> MGETKKMICLVDGEHYFPVVKDSIEILDDLEHIDVVAVVFIGGTEKLQIEDPKEYSEKLGKPVFFGPDPKKIPYDVIKKCVKKYNADIVMDLSDEPVVDYTKRFRIASIVLKEGAVYQGADFKFEPLTEYDVLEKPSIKIIGTGKRIGKTAVSAYAARVIHKHKYNPCVVAMGRGGPREPEIVEGNKIEITAEYLLEQADKGVHAASDHWEDALMSRILTVGCRRCGGGMLGDTFITNVKRGAEIANKLDSDFVIMEGSGAAIPPVKTNRQIVTVGANQPMININNFFGPFRIGLADLVIITMCEEPMATTEKIKKVEKFIKEINPSANVIPTVFRPKPVGNVEGKKVLFATTAPKVVVGKLVNYLESKYGCDVVGVTPHLSNRPLLRRDLKKYINKADLMLTELKAAAVDVATRVAIEAGLDVVYCDNIPVVIDESYGNIDDAIIEVVEMAIDDFKNNR

The enzyme cyclic di-phosphoglycerate synthetase that is involved in the production of the osmolyte cyclic 2,3-diphosphoglycerate has been studied both biochemically and structurally. The reaction involves the transfer of the γ-phosphate group from ATP to the substrate 2,3 -diphosphoglycerate and the subsequent SN2 attack to form a phosphoanhydride. The unique structure of cDPGS is made up of an N-terminal domain which is crucial for the stabilization of the active dimeric structure and the ligand interactions, and a C-terminal domain that contains a P-loop kinase fold as part of its structure. Since the cDPGS reaction is exergonic at cellular concentrations, cDPG accumulation is favored thermodynamically until this reaction reaches equilibrium. cDPG appears to play a role in the thermoprotection of proteins, and increased thermostability has been demonstrated for several model enzymes in its presence.

The cDPGS crystallized readily in many screening conditions and the structure of the apo-cDPGS was solved by the single wavelength anomalous dispersion (SAD) method using data collected from a selenomethionine protein crystal. The space group was determined to be I222 with a single protomer of cDPGS in the asymmetric unit. The structure was refined to 1.7 Å resolution and was found to contain the entire polypeptide chain. This has been refined to R and Rfree values of 17.7 and 21.3%, respectively. The structure of cDPGS can be split into two domains. The smaller N-terminal domain contains a six-stranded β-sheet of mixed type with direction + + + + + − and connectivity -1x,-1x,3x,1x,1 flanked by 4 α-helices (α1–α4). The β-sheets of the two N-terminal domains in the cDPGS dimer form a large intersubunit 12 strand β-sheet on the molecular dyad. The larger C-terminal domain (residues 136–460) contains a twelve-stranded β-sheet (β7 – β18) surrounded by twelve α-helices. The cDPGS structure shows a tight dimer that buries a surface area of 2844.1 Å2, accounting for 13.7% of the total solvent accessible area of the protomer. The interface is stabilized by 36 hydrogen bonds and 24 salt bridges between the interacting subunits as estimated by PISA.> MNENEPVSIWMHPEPAGRRSARSHRTLSRDQIVRAAVKVADTEGVEAASMRRVAAELGAGTMSLYYYVP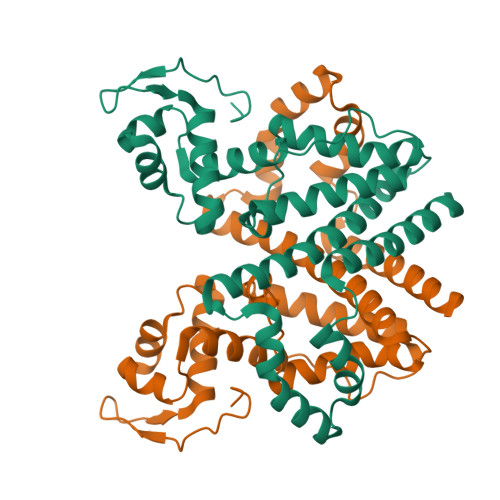TKEDLVELMVDEVIGETRLPDRPGPDWRAALTLAANEKRALWLRHPWLATAWRNGHPVWGPNSLRQQEFVLGTLGVFDLQVDELLSLIGLYNGYVESFVRNEVGWLEEARRTKVDMREWMRRSGPYAQQLVDSGEYPMFARVLAETVAPHMGPDQRFRSGLERLLDSIGASLDRLSPPGRSAASERPALALEHHHHHH>[4x]XM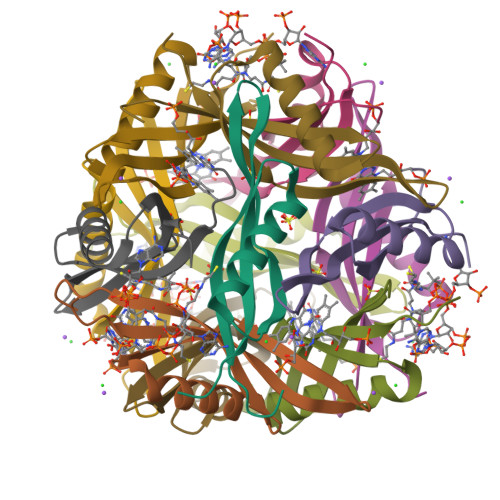SNHTYRVTEVVGTSPDGVDQAVRNAVTRASQTLRKLDWFEVTQVRGQIEDGQVAHWQVGLKLGFRLEES>[4x]TKNPQLPTQDELKHKSKPAQSFNNDVNQKDTRATSLFETDPSISNNDDSGQFNVVDSKDTRQFVKSIAKDAHRIGQDNDIYASVMIAQAILESDSGRSALAKSPNHNLFGIKGA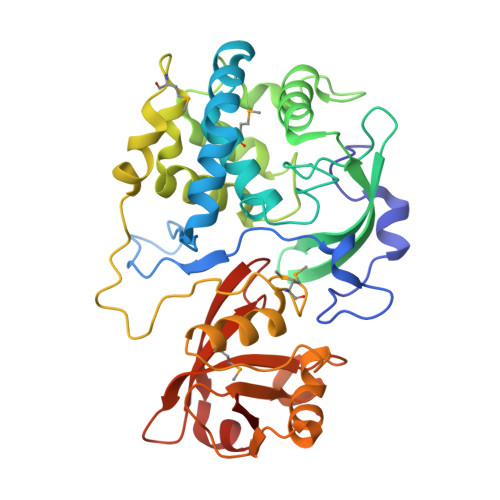FEGNSVPFNTLEADGNQLYSINAGFRKYPSTKESLKDYSDLIKNGIDGNRTIYKPTWKSEADSYKDATSHLSKTYATDPNYAKKLNSIIKHYQLTQFDDERMPDLDKYERSIKDYDDSSDEFKPFREVSDSMPYPHGQCTWYVYNRMKQFGTSISGDLGDAHNWNNRAQYRDYQVSHTPKRHAAVVFEAGQFGADQHYGHVAFVEKVNSDGSIVISESNVKGLGIISHRTINAAAAEELSYITGK> VIVPEGTQLDEKQHIVINNGAEPQSFDPHKTEGVPESNVAYQLLEGLVTSDSEGKLQPGAAESWENTPDFKTWTFHLRKDAKWSNGDPVTAHDFVFAWRRLVDPATAAPYASYLSYLQVENAQDIIDGKKKPAELGVEAKDDYTFVVHATNPVPYAVSLTTHQSLLPLPQKVVEKLGDAWVKKENYVGNGAYKLANHIINEKIEFERNPLYWNDKETVINSATFLAIENPSTDVARYRAGDLDMTSYGLPPEQFAKLKKELLGEVYVTRTLGTYSYELNNKKAPFDNVNIRKALNL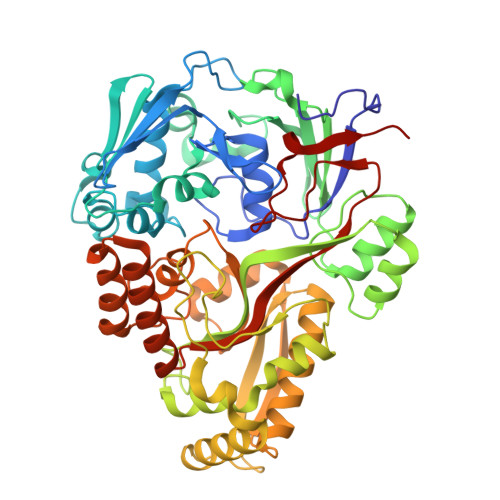SLDRNVITDKVLGQGQTPTYVFTPTYIEEGHLIQQPAYSKEPMAQRNEEAIKLLEEAGYSKANPLKFSILYNTNENHKKVAIAAASMWKANTKGLIDVKLENQEWKTYIDSRRAGRYDVARAGWHADYNQATTFGNYFLSNSSNNTAKYANPEYDKAMAESYAATDAEGRAKAYAKAEEILGKDYGIVPIFNYVNPRLVKPYVKGYSGKDPQDHIYLRNLYIIKH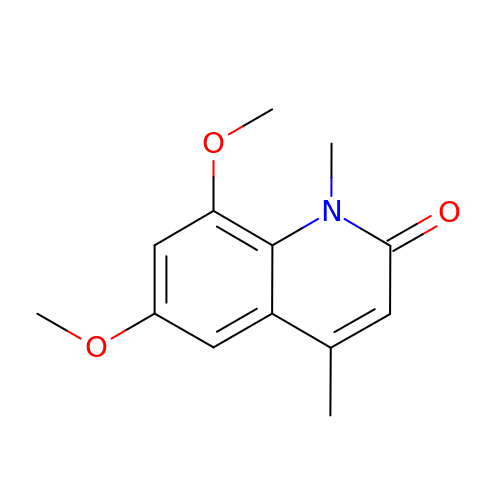6,8-dimethoxy-1,4-dimethylquinolin-2(1H)-one | C13 H15 N O3 | BYYQQWLTZFBHIQ-UHFFFAOYSA-N> MSTAKAPTLPASIFRAYDIRGVVGDTLTAETAYWIGRAIGSESLARGEPCVAVGRDGRLSGPELVKQLIQGLVDCGCQVSDVGMVPTPVLYYAANVLEGKSGVMLTGSHNPPDYNGFKIVVAGETLANEQIQALRERIEKNDLASGVGSVEQVDILPRYFKQIRDDIAMAKPMKVVVDCGNGVAGVIAPQLIEALGCSVIPLYCEVDGNFPNHHPDPGKPENLKDLIAKVKAENADLGLAFDGDGDRVGVVTNTGTIIYPDRLLMLFAKDVVSRNPGADIIFDVKCTRRLIALISGYGGRPVMWKTGHSLIKKKMKETGALLAGEMSGHVFFKERWFGFDDGIYSAARLLEILSQDQRDSEHVFSAFPSDISTPEINITVTEDSKFAIIEALQRDAQWGEGN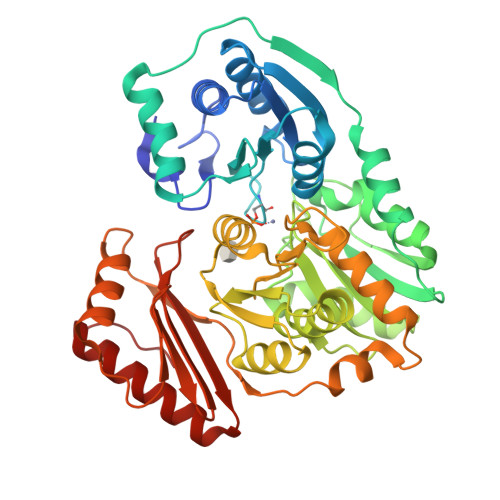ITTLDGVRVDYPKGWGLVRASNTTPVLVLRFEADTEEELERIKTVFRNQLKAVDSSLPVPF Sulfinpyrazone 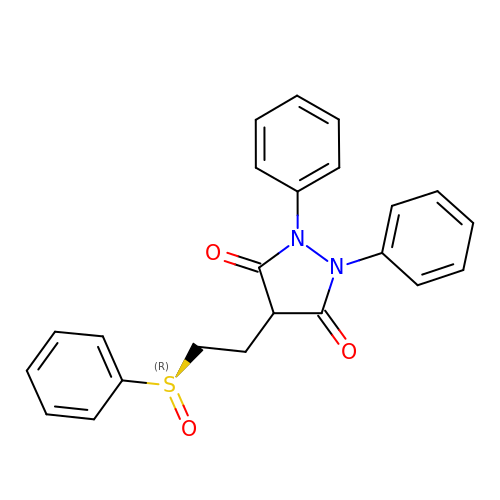| C23 H20 N2 O3 S | MBGGBVCUIVRRBF-UHFFFAOYSA-N RIBAVIRIN TRIPHOSPHATE | C8 H15 N4 O14 P3 | 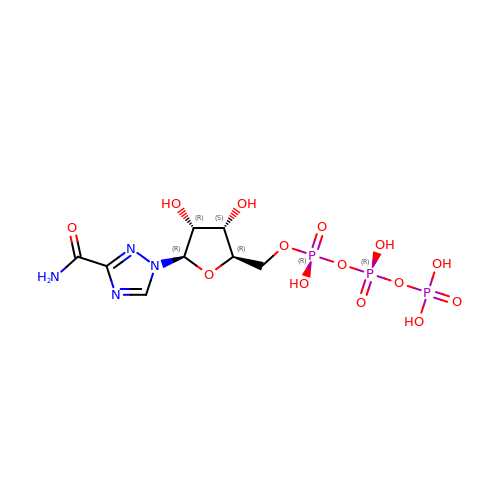MMJOCKKLRMRSEQ-AFCXAGJDSA-N>DEDEDDLQRYIDVTRGELFFARGIIFVEGDAERFLIPAFAEALDIHLDILGISVCSVSGTNFAPYIKLVGPTGLNIPHVVLTDLDPVDDRPPLARKRLLRLLELAVTDEEWDELDEDEPWDLGEEYGYFVNDSTLEPELFQAGLGSGIRDVIESELSTSAQTREALACWVDDPTALNNERLLKLIERIGKGRFAQALAGFATADTCPAYIRNALEYIRDAVALEHHHHHH[2x]

Overcoming lysogenization defect (OLD) proteins constitute a family of uncharacterized nucleases present in bacteria, archaea, and some viruses. These enzymes contain an N-terminal ATPase domain and a C-terminal Toprim domain common amongst replication, recombination, and repair proteins. Here we identify and define two classes of OLD proteins based on differences in gene neighborhood and amino acid sequence conservation and present the crystal structures of the catalytic C-terminal regions from the Burkholderia pseudomallei and Xanthamonas campestris p.v. campestris Class 2 OLD proteins at 2.24 Å and 1.86 Å resolution respectively. The structures reveal a two-domain architecture containing a Toprim domain with altered architecture and a unique helical domain.

Crystals of the analogous BpCTR construct diffracted to a slightly lower resolution (2.2–2.3 Å) but produced a more complete structural model (residues 390–594). BpCTR contains two domains: a Toprim domain (residues 390–504, purple) and a unique helical domain (residues 505–594, yellow) consisting of a five-helix orthogonal bundle and an additional C-terminal amphipathic helix (α6H). α6H extends into a groove along one face of the Toprim's central β-sheet, forming extensive hydrophobic interactions. BpCTR crystallized in a different space group thereby permitting the helical domain to rotate and scrunch closer to the Toprim domain. Consequently, T506 and E508 shift 1.2 and 1.5 Å toward the active site respectively, which facilitates the binding of two magnesium ions in a geometry consistent with two metal catalysis. Each magnesium is octahedrally coordinated with a water molecule bridging the two metals where the scissile phosphate would normally sit. The metals are spaced 4.9 Å apart, suggesting they may move closer together once DNA is engaged. The conserved Toprim glutamate (E400) and the first aspartate of the DxD motif (D455) each provide a ligand to the first magnesium (metal A). E508, located in αH1 of the helical domain, directly coordinates the second magnesium (metal B), while E404 and T506 stabilize additional metal B waters. We also identify a conserved lysine residue in α5H (K562) that extends toward the active site, separated from metal A by 5.5 Å and from metal B by 3.8 Å. Mutant combinations of either the metal A or the metal B interacting residues together completely abolish Bp OLD nuclease activity on linear DNA substrates in vitro.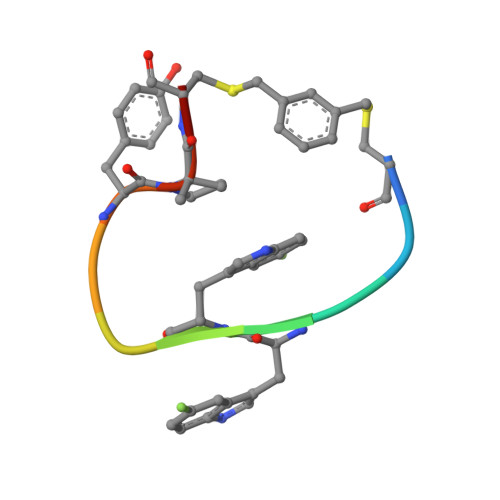> XKGWWDHYXCA> MNKQIFVLYFNIFLIFLGIGLVIPVLPVYLKDLGLTGSDLGLLVAAFALSQMIISPFGGTLADKLGKKLIICIGLILFSVSEFMFAVGHNFSVLMLSRVIGGMSAGMVMPGVTGLIADISPSHQKAKNFGYMSAIINSGFILGPGIGGFMAEVSHRMPFYFAGALGILAFIMSIVLIHDPKKSTTSGFQKLEPQLLTKINWKVFITPVILTLVLSFGLSAFETLYSLYTADKVNYSPKDISIAITGGGIFGALFQIYFFDKFMKYFSELTFIAWSLLYSVVVLILLVFANDYWSIMLISFVVFIGFDMIRPAITNYFSNIAGERQGFAGGLNSTFTSMGNFIGPLIAGALFDVHIEAPIYMAIGVSLAGVVIVLIEKQHRAKLKEQNMENLYFQGKLGPEQKLISEE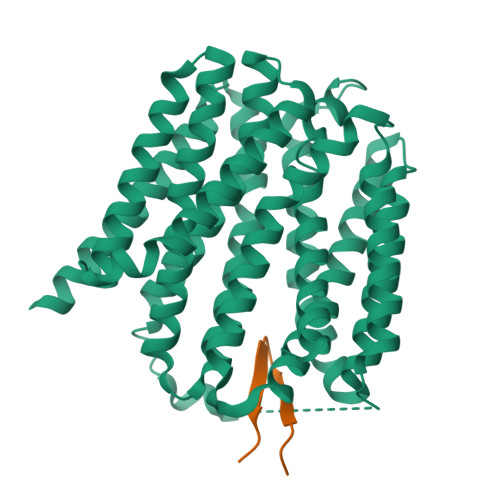DLNSAVDHHHHHHHHHH;> SVENHWYYFYWYMSP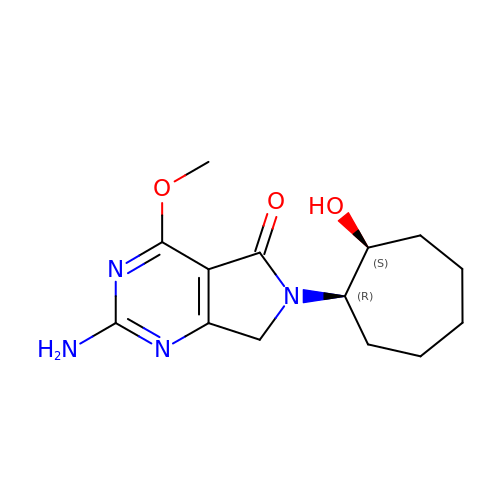2-azanyl-4-methoxy-6-[(1~{R},2~{S})-2-oxidanylcycloheptyl]-7~{H}-pyrrolo[3,4-d]pyrimidin-5-one | C14 H20 N4 O3 | DXJAJOUDYQSXQN-YHMJZVADSA-N>[2x]HHHHHHENLYFQGSGSSPRSGVLLRGCPTHCHCEPDGRMLLRVDCSDLGLSELPSNLSVFTSYLDLSMNNISQLLPNPLPSLRF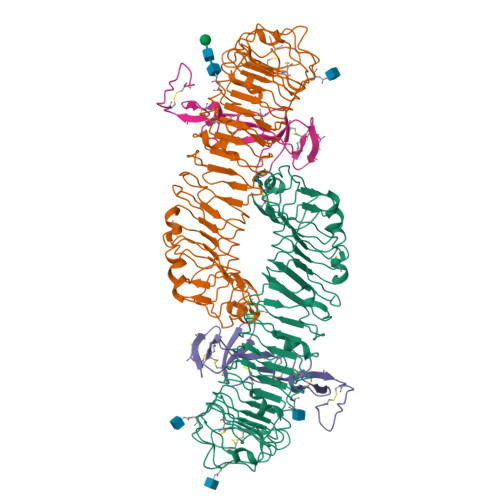LEELRLAGNALTYIPKGAFTGLYSLKVLMLQNNQLRHVPTEALQNLRSLQSLRLDANHISYVPPSCFSGLHSLRHLWLDDNALTEIPVQAFRSLSALQAMTLALNKIHHIPDYAFGNLSSLVVLHLHNNRIHSLGKKCFDGLHSLETLDLNYNNLDEFPTAIRTLSNLKELGFHSNNIRSIPEKAFVGNPSLITIHFYDNPIQFVGRSAFQHLPELRTLTLNGASQITEFPDLTGTANLESLTLTGAQISSLPQTVCNQLPNLQVLDLSYNLLEDLPSFSVCQKLQKIDLRHNEIYEIKVDTFQQLLSLRSLNLAWNKIAIIHPNAFSTLPSLIKLDLSSNLLSSFPITGLHGLTHLKLTGNHALQSLISSENFPELKVIEMPYAYQCCAFGVCENAYKISNQWNKGDNSSMDDLHKKDAGMFQAQDERDLEDFLLDFEEDLKALHSVQCSPAAA;>[2x]GSRISAEGSQACAKGCELCSEVNGCLKCSPKLFILLERNDIRQVGVCLPSCPPGYFDARNPDMNKCIKCKIEHCEACFSHNFCTKCKEGLYLHKGRCYPACPEGSSAANGTMECSSPAAAHHHHHH> MGSSHHHHHHGSGENLYFQSNQPLKIVVPFSAGGTADVLPRLVAEKIRADYAGGVIIENKPGAGGNIGADLVFRAPPDGMTVLASPPGPIAINHNLYQKLSFDPTRWVPVTILATVPNVLVINPKLPVKSLGEFIAYAKANPKKVTVATQGDGSTSHLTAAMFMQLTGTELTVIPYKGTAPALIDLIGGNVDVFFDNISSSATYHQAGKVRILAVADEQRSQILPQVPTFAEQQWPAMQAVTFFSVVAPPGTSAEIAQKLQKQMALALSSNDIRKHFQEQGAVPCGWDPSKTAQFIRQETEKWKKVLKAANVKL

In this study, we characterised the TphC SBP that is a key component in the cellular uptake of TPA, the breakdown product of PET plastic. TphC belongs to the TTT family in Commamonas sp. strain E6 and through biochemical and structural analysis, the ligand-binding properties and 3D structure were determined in both open and ligand-bound closed forms. As with the tripartite ATP-independent periplasmic (TRAP) class of SBP-dependent transporters, they are symporter proteins driven by an electrochemical ion-gradient, rather than ATP as per the SBP-dependent class of ABC transporters. Here, we report the biochemical and structural characterisation of TphC in both open and TPA-bound closed conformations. This analysis demonstrates the narrow ligand specificity of TphC towards aromatic para-substituted dicarboxylates, such as TPA and closely related analogues.

Purified TphC was readily co-crystallised in the presence of 2 mM TPA and crystals diffracted to 2.4 Å resolution. The general architecture of the previously reported TTT-SBPs is maintained in the TphC–TPA structure. Superposition of the open and closed TphC structures highlights an ~36° closure between the two domains upon TPA binding. Upon closure the solvent accessible surface area of TphC decreases from 13,048 to 12,495 Å2 encapsulating a closed cavity of 280 Å3 in which the TPA is bound. The bound TPA is recognised through a number of direct and water-mediated hydrogen bond interactions. The TPA carboxylate group buried deepest within the pocket is recognised and stabilised through direct (T155, T242) and water-mediated hydrogen bonds (T155, Q150, N197). The second carboxyl group of the TPA hydrogen bonds to the backbone amino groups of A36 and with additional water-mediated interactions with the backbones of G34, S31 and T179. The interactions at this second carboxylate group span between the two TphC domains stabilising the closed conformation. The binding pocket is bordered on one side by a conserved aromatic residue (F30); the positioning of this sidechain is facilitated by the proximity of a conserved glycine (G178). Unlike other TTT-SBPs characterised to date, the ligand site of TphC contains bulky amino acids P86 and Q150, the sidechains of which create a very narrow pocket 6.4 Å across, which would appear to confer the observed selectivity toward planar aromatic ligands.>[2x]MQIKVNDNEFQLFVGEKRILEHSKERPMIYVGVGQEDVDMYRGNFKITDYVTERFPLKLTDVIQTADTVRLCFESYIIAKIKCDENLCTIDFEQKDDRINRFWFRVAADKEEKCYGCGEQMSYFNLRGRNFPIWTSEPGVGRDKTTYVTWRSDVENKAGGDYYNTNYPQPTFVSTNKYYLHVDSTAYADFDFRNDSFHELQIWEVPKQIRIECADTYLKLLERITTYFGRQPKLPDWVYNGLIIGVQGGN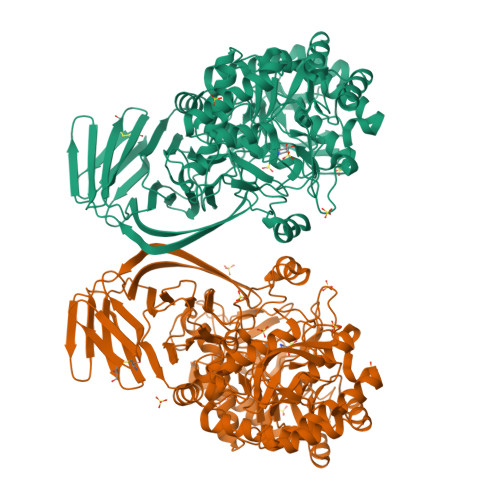ERSFGLLDKTLDRNIKVAGIWCQDWCGKRVTSFGKRLQWDWKYHKEMYPDLPKKIKEINAKGIKFLGYVNPYLVNDGELYKEGKEKGYFATKADGSDYLVDFGEFYCGVVDLTNPEAFEWFKDIIKEYTLGIGIDGWMADFGEYLPTDDICLYSGKSPMIEHNHWPVLWAKCNYEAVKESGKLGDVVYFMRAGGAGSQKYCTLLWAGDQSVDFTIHDGLASVICGALSAGMMGCGLTHSDIGGYTSLFDNTRTKELFLRWAEMAMFTPFMRTHEGNRPDTNFQYYDDEDTMERLARLVDVYTMLAPYTKTLVEENADSGHPVQRPLFMHYESDAKAYDIQYEYLFGRDMLIAPVYEQDKHEWDVYLPQDEWVHLWTGEEYHGGEITVSAELGYTPAFYRKNSEFADIFEEIREKYGVKLEHHHHHH> GSHMLEDPLRVSPMIREFVQSIDDREWQTQLFALLQKQTYNQVEVDLFELMCKVLDQNLFSQVDWARNTVFFKDLKVDDQMKLLQHSWSDMLVLDHLHHRIHNGLPDETQLNNGQVFNLMSLGLLGVPQLGDYF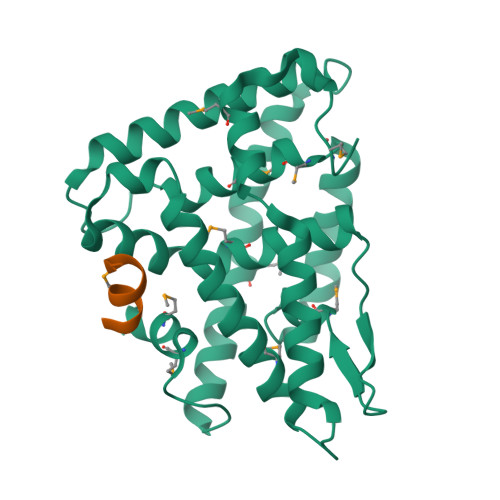NELQNKLQDLKFDMGDYVCMKFLILLNPSVRGIVNRKTVSEGHDNVQAALLDYTLTCYPSVNDKFRGLVNILPEIHAMAVRGEDHLYTKHCAGSAPTQTLLMEMLHAKRKG;> STLRALLTN>MPYRNCWSKIMKKLINDVQDVLDEQLAGLAKAHPSLTLHQDPVYVTRADAPVAGKVALLSGGGSGHEPMHCGYIGQGMLSGACPGEIFTSPTPDKIFECAMQVDGGEGVLLIIKNYTGDILNFETATELLHDSGVKVTTVVIDDDVAVKDSLYTAGRRGVANTVLIEKLVGAAAERGDSLDACAELGRKLNNQGHSIGIALGACTVPAAGKPSFTLADNEMEFGVGIHGEPGIDRRPFSSLDQTVDEMFDTLLVNGSYHRTLRFWDYQQGSWQEEQQT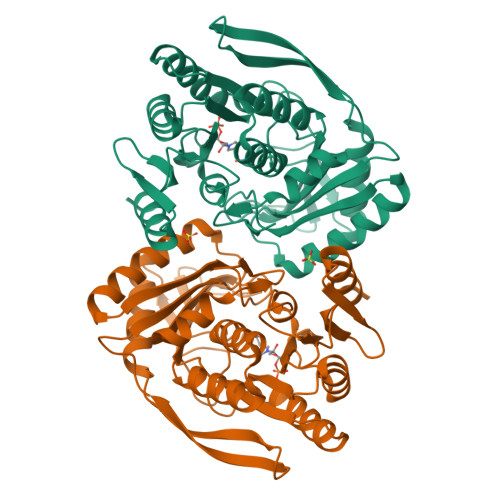KQPLQSGDRVIALVNNLGATPLSELYGVYNRLTTRCQQAGLTIERNLIGAYCTSLDMTGFSITLLKVDDETLALWDAPVHTPALNWGK[2x]NAPHTHALEN-2-YL-3-ALANINE 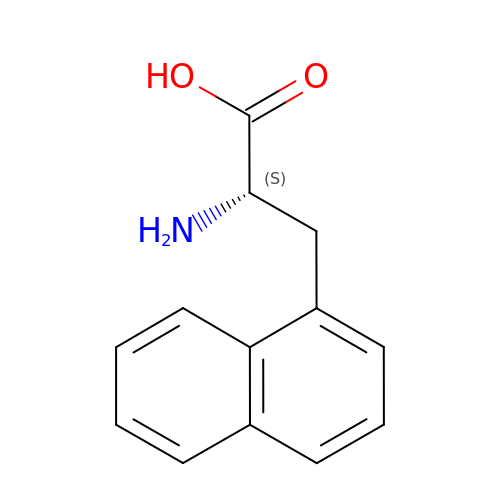| C13 H13 N O2 | OFYAYGJCPXRNBL-LBPRGKRZSA-N>GSHMVVKFTDSQIQHLMEYGDNDWSEAEFEDAAARDKEFSSQFSKLKSANDKGLKDVIANPRNDLTDLENKIREKLAARGFIEVHTPIFVSKSALAKMTITEDHPLFKQVFWIDDKRALRPMHAMNLYKVMRELRDHTKGPVKIFEIGSCFRKESKSSTHLEEFTMLNLVEMGPDGDPMEHLKMYIGDIMDAVGVEYTTSREESDVYVETLDVEINGTEVASGAVGPHKLDPAHDVHEPWAGIGFGLERLLMLKNGK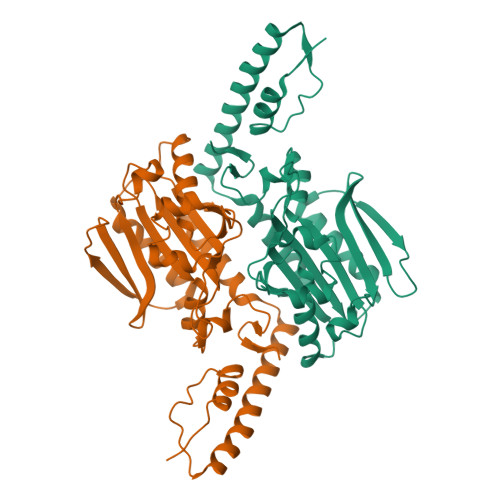SNARKTGKSITYLNGYKLD[10x]> MIFLLLMLSLELQLHQIAALFTVTVPKELYIIEHGSDVTLECNFDTGSHVNLGAITAS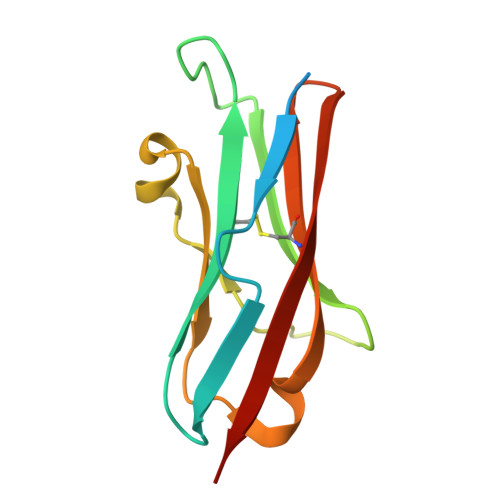LQKVEDDTSPHRERATLLEEQLPLGKASFHIPQVQVRDEGQYQCIIIYGVAWDYKYLTLKVKASY Human thymidylate synthase (hTS) is an obligate, stable homodimer (Kd = 80 nM Genovese et al., 2010) with two active sites, each including residues from both monomers. As a dimeric enzyme, it provides the sole de novo pathway to deoxythymidylate (dTMP) synthesis in human cells by catalyzing the reductive methylation of deoxyuridylate (dUMP) to dTMP using methylenetetrahydrofolate (mTHF) as the one-carbon methyl donor. By interacting with its own and other mRNAs, this protein regulates its own levels and those of other proteins involved in apoptotic processes, including bcl2, c-myc, and p53. Its inhibition is usually achieved with compounds that bind at the protein active-site, competing either with the dUMP substrate, such as 5-fluorodeoxyurdine 5’-monophosphate (FdUMP), or with the folate cofactor, such as raltitrexed (RTX) and pemetrexed (PMX) (Carreras and Santi, 1995; Jennings and Willis, 2015). Here we report the discovery of molecules that bind at the hTS monomer/monomer interface and, despite their small size, markedly shift the monomer-dimer equilibrium of the enzyme towards the inactive monomeric form.

We selected the ‘Y202 pocket’, which accommodates the side chain of F59’ from the other monomer, as the most promising region to target (Salo-Ahen et al., 2015). We therefore made the Y202C mutant and screened for compounds able to form a covalent disulfide bond with C202 from a library of organic disulfides. We made mutants with single point mutations at C195S and Y202C to test their functional and structural properties as well as the double mutant, hTS C195S-Y202C. Panel (c) reports the omit map (contoured at 3.0 σ) showing the S,S(2-hydroxyethyl)cysteine (CME) chemical modification occurring at the mutated residue C202 in the single hTS Y202C mutant. (d-e) H-bond interactions (represented as dashed lines) involving the CME202 residue in hTS Y202C subunits A and B. (f–g) two views of the surface of the hTS Y202C dimer. The two symmetry-related subunits are shown in violet (subunit A) and orange (subunit B), while the CME and S-methyl-thio-cysteine (SCH) residues are represented as spheres. Only SCH43, appears fully solvent accessible, with CME202, partially visible in its pocket, just below SCH43. Panel (g) shows that SCH180 is partially solvent accessible, while SCH195, CME199, and C210 are buried to different extents below the hTS surface. Four molecules, A5, A10, A20, and TPC also bound peptide (D186-R215) DLPLMALPPSHALCQFCVVNSELSCQLYQR (sequence C), containing the engineered Y202C together with the native C199 and C210. In agreement with the described computational and crystallographic data (see above), Y202C is the most exposed of these three cysteines and is thus easily available for disulfide-bond formation with the RS fragments, being therefore suitable for tethering experiments.

>[2x]MRGSHHHHHHGSMPVAGSELPRRPLPPAAQERDAEPRPPHGELQYLGQIQHILRCGVRKDDRTGTGTLSVFGMQARYSLRDEFPLLTTKRVFWKGVLEELLWFIKGSTNAKELSSKGVKIWDANGSRDFLDSLGFSTREEGDLGPVYGFQWRHFGAEYRDMESDYSGQGVDQLQRVIDTIKTNPDDRRIIMCAWNPRDLPLMALPPCHALCQFCVVNSELSCQLYQRSGDMGLGVPFNIASYALLTYMIAHITGLKPGDFIHTLGDAHIYLNHIEPLKIQLQREPRPFPKLRILRKVEKIDDFKAEDFQIEGYNPHPTIKMEMAV> MPPGKCLFSGVFCNMAEKQTAKRNRREEILQSLALMLESSDGSQRITTAKLAASVGVSEAALYRHFPSKTRMFDSLIEFIEDSLITRINLILKDEKDTTARLRLIVLLLLGFGERNPGLTRILTGHALMFEQDRLQGRINQLFERIEAQLRQVLREKRMREGEGYATDETLLASQILAFCEGMLSRFVRSEFKYRPTDDFDAR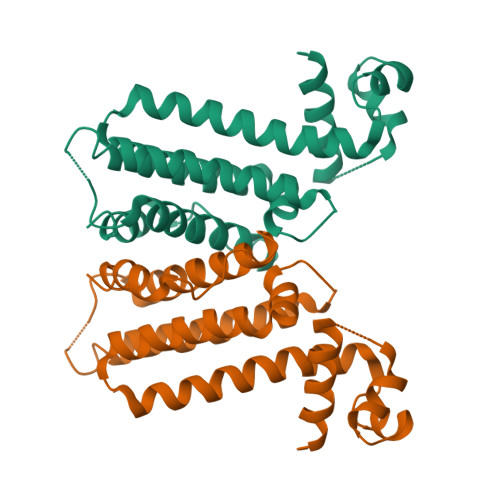WPLIAAQLQ5-bromanyl-2-(2-fluoranylpyridin-4-yl)-1,7-naphthyridin-8-amine | 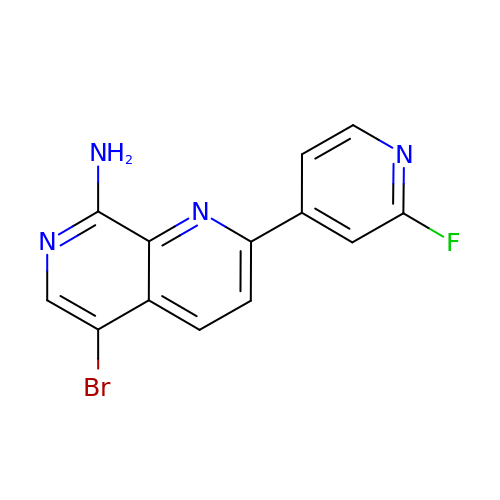C13 H8 Br F N4 | KARJFNUGCLEZKM-UHFFFAOYSA-N> MSVLQVLHIPDERLRKVAKPVEEVNAEIQRIVDDMFETMYAEEGIGLAATQVDIHQRIIVIDVSENRDERLVLINPELLEKSGETGIEEGCLSIPEQRALVPRAEKVKIRALDRDGKPFEL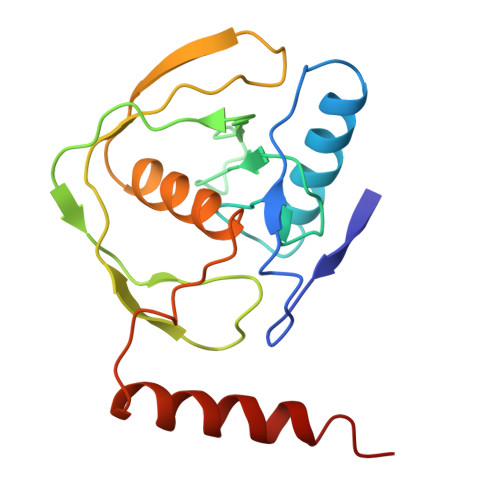EADGLLAICIQHEMDHLVGKLFMDYLSPLKQQRIRQKVEKLDRLKARA> SASRDDWRAARSMHEFSAKDID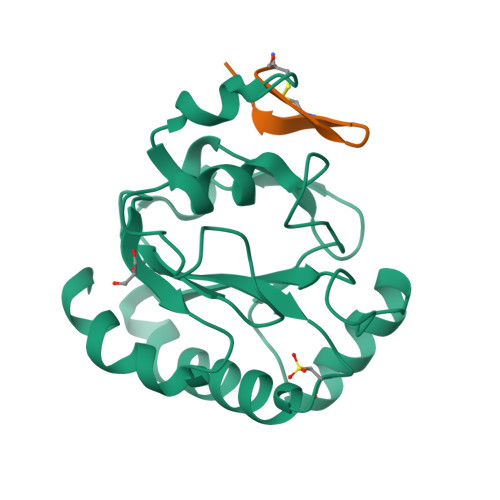GHMVNLDKYRGFVSIVTNVASQCGKTEVNYTQLVDLHARYAERGLRILAFPSNQFGKQEPGSNEEIKEFAAGYNVKFDMFSKIEVNGDDAHPLWKWMKIQPKGKGILGNAIKWNFTKFLIDKNGVVVKRYGPMEEPLVIEKDLPHYF;> XCRAWYQNYCALRRX Centrioles are complex microtubule (MT) based structures that are required for the formation of centrosomes and cilia/flagella. The protein kinase recruits STIL/Ana2/SAS-5 and Sas-6 to a single site on the side of the mother centriole where they assemble with CPAP/Sas-4 into a cartwheel structure that helps to establish the ninefold symmetry of the centriole. Here we show that Ana2/STIL proteins also homo-oligomerise and that mutations that perturb the homo-oligomerisation of fly Ana2 in vitro also strongly perturb centriole assembly in vivo. Thus, Sas-6 homo-oligomerisation alone appears unable to drive efficient cartwheel assembly in vivo if Ana2 is unable to homo-oligomerise.

To test this possibility, we bacterially expressed and purified the 37aa CCCD region (residues 193–229)—as predicted by the COILS server —as a His-tagged diLipoyl peptide. A SEC-MALS analysis revealed that the purified protein, either with or without the Lipoyl tags, formed a tetramer at a wide range of concentrations (36–900 μM). The purified Ana2 CCCD protein readily formed protein crystals that diffracted extremely well, enabling us to refine a structure to 0.80 Å resolution. The structure demonstrated that the Ana2 CCCD forms a parallel, symmetrical 4-helix bundle, with a left-handed supercoil. This structure appears to be unusual as we could find only one other natural soluble protein in the PDB that homo-tetramerises through a parallel four-helical bundle (NSP4, a tetrameric enterotoxin secreted by rotaviruses). Analysis using the PISA server showed that residues located at the g, a, d and e positions of the helical heptad repeat were all buried at the tetramer interface (yellow residues). (D) A transverse N-C view of a QQQ triad which adopts positions g, a and b of the heptad. These polar side-chains form an inward facing hydrogen-bond network. We replaced all ten residues at the d and g positions of the CCCD with either Ala (CCCD-A), Ser (CCCD-S) or Asp (CCCD-D) (residues circled in red). A SEC-MALS analysis revealed that all of these mutant CCCD proteins behaved as monomers rather than tetramers in vitro. Thus, in flies, the Ana2 CCCD parallel tetramer tethers the CR2 and STAN domains in a particular geometry and stoichiometry.

> GGSNKSDLAALVSLVESVRHEQQQLRNLCEMILEQQQRAKEFGENLYFQ> MGSSHHHHHHSSGTGSGENLYFQGHMKSDFKFSNLLGTVYRQGNITFSDDGKQLLSPVGNRVSVFDLINNKSFTFEYEHRKNIAAIDLNKQGTLLISIDEDGRAILVNFKARNVLHHFNFKEKCSAVKFSPDGRLFALASGRFLQIWKTPDVNKDRQFAPFVRHRVHAGHFQDITSLTWSQDSRFILTTSKDLSAKIWSVDSEEKNLAATTFNGHRDYVMGAFFSHDQEKIYTVSKDGAVFVWEFTKRPSDDDDNESEDDDKQEEVDISKYSWRITKKHFFYANQAKVKCVTFHPATRLLAVGFTSGEFRLYDLPDFTLIQQLSMGQNPVNTVSVNQTGEWLAFGSSKLGQLLVYEWQSESYILKQQGHFDSTNSLAYSPDGSRVVTASEDGKIKVWDITSGFCLATFEEHTSSVTAVQFAKRGQVMFSSSLDG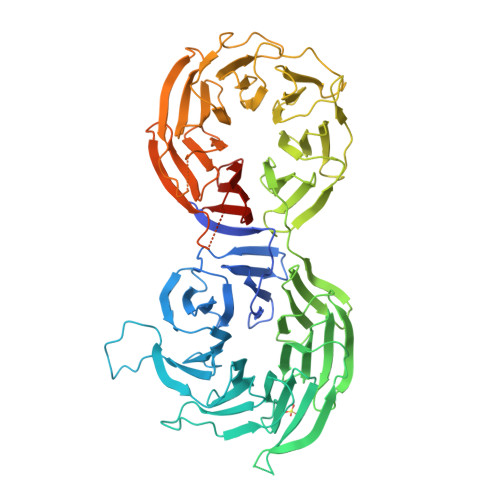TVRAWDLIRYRNFRTFTGTERIQFNCLAVDPSGEVVCAGSLDNFDIHVWSVQTGQLLDALSGHEGPVSCLSFSQENSVLASASWDKTIRIWSIFGRSQQVEPIEVYSDVLALSMRPDGKEVAVSTLKGQISIFNIEDAKQVGNIDCRKDIISGRFNQDRFTAKNSERSKFFTTIHYSFDGMAIVAGGNNNSICLYDVPNEVLLKRFIVSRNMALNGTLEFLNSKKMTEAGSLDLIDDAGENSDLEDRIDNSLPGSQRGGDLSTRKMRPEVRVTSVQFSPTANAFAAASTEGLLIYSTNDTILFDPFDL>[4x]MCTTYTIKSGDTCYAISQ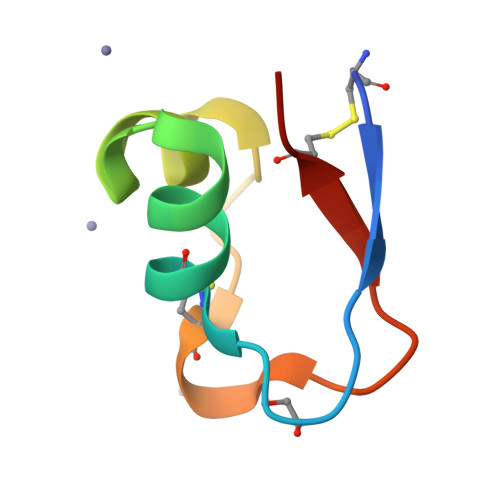ARGISLSDFESWNAGIDCNNLQIGQVVCVSK(9E)-OCTADEC-9-ENAMIDE 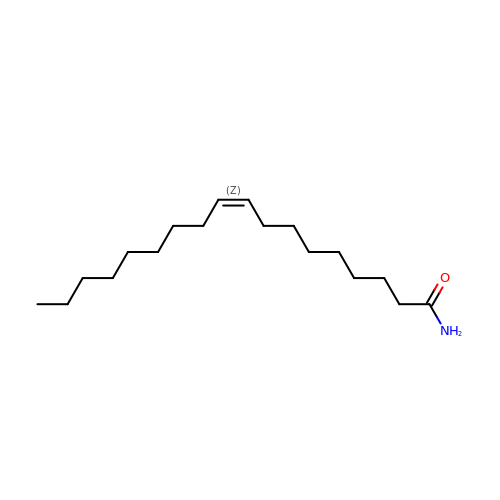| C18 H35 N O | FATBGEAMYMYZAF-UHFFFAOYSA-N>[2x]MTEKLNEIVVRKTKNVEDHVLD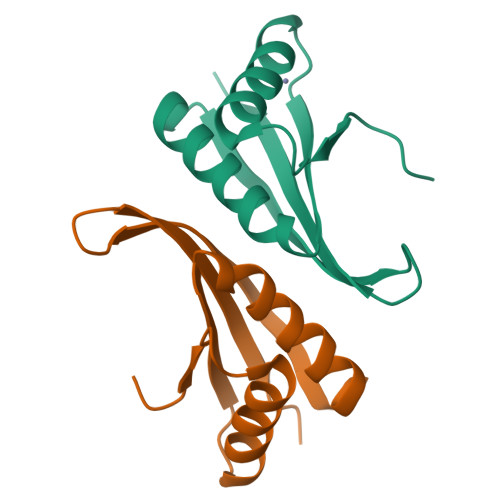VIVLFNQGIDEVILKGTGREISKAVDVYNSLKDRLGDGVQLVNVQTGSEVRDRRRISYILLRLKRVY(2~{R})-2-[(4~{S})-6-(4-chlorophenyl)-9-methoxy-1-methyl-4~{H}-[1,2,4]triazolo[4,3-a][1,4]benzodiazepin-4-yl]-~{N}-ethyl-propanamide | C23 H24 Cl N5 O2 | 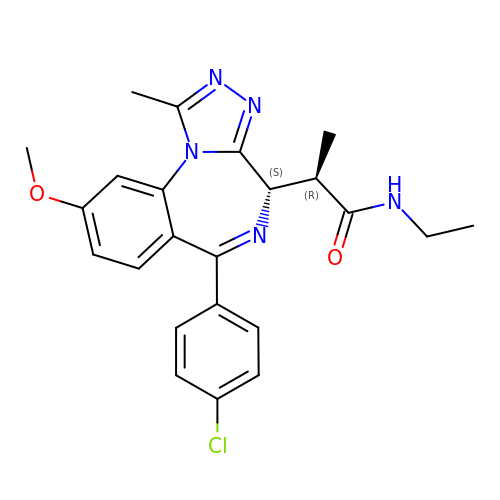SWPWVZYAERLDQC-XCLFUZPHSA-N2-[1-methyl-5-[[1-[3-(pyrimidin-2-ylamino)phenyl]carbonylpiperidin-4-yl]amino]-1,2,4-triazol-3-yl]-1~{H}-indole-6-carbonitrile 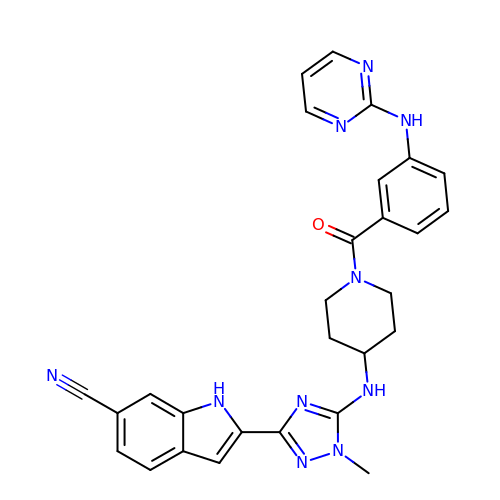| C28 H26 N10 O | MFOILUADHAWEJH-UHFFFAOYSA-N>[2x]GSHMDSEIQMENLVERKHHRLARSERSGISDRDAKPTASIRDQLHTIVYRYPPTYVLSSEEQDLVWKFRFYLSSHKKALTKFLKCINWKLEDEVTQALWMLANWAPMDVEDALELLSPTFTHPQVRKYAVSRLAQAPDEDLLLYLLQLVQALKYEDPRHIVHLHGCIFPERDVVRSILDDNGSLLDQSSLSDLSATSSGLHASVIPANQRA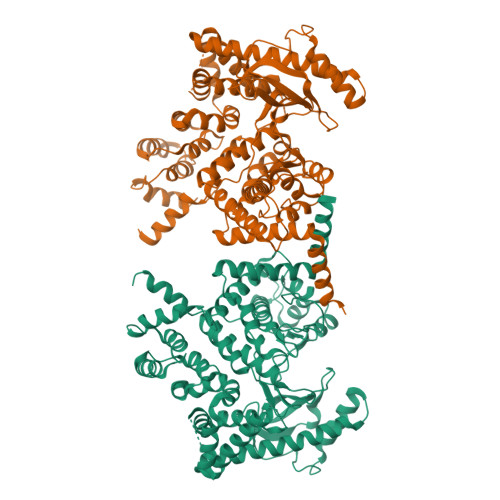ASVLAAIKSDKSVSPGSAGGSGSGGQGSVALPNPSAPATPGSSSLPCDSNSNALMLAEGISFGSVPANLCTFLIQRACTNATLANYFYWYLSIEVEEVESVRKQDERAHDMYAMVLKMFLKVLENGNFNLRGIFYNLRKQRRFIDELVKLVKLVAKEPGNRNKKTEKFQKLLAEQDMFKVNFTNFEPIPFPLDPEIYITKIVPMRTSLFKSALMPAKLTFVTSIAHHEYAAIFKHGDDLRQDQLILQMITLMDKLLRRENLDLKLTPYKVLATSSKHGFLQYVDSCTVAEVLAREGNIHNFFRKHHPCDNGPYGISAEVMDTYIKSCAGYCVITYLLGVGDRHLDNLLLTTNGKLFHIDFGYILGRDPKPMPPPMKLSKEMVEAMGGISSEHHHEFRKQCYTAYLHLRRHANVMLNLFSLMVDATVPDIALEPDKAVKKVEENLQLGLTDEEAVQHLQSLLDVSITAVMPALVEQIHRFTQYWRK> STLSPNASVFKP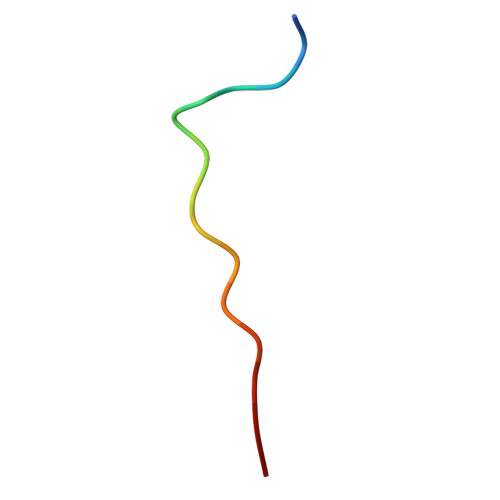SRS> MSSIIRKIINTSKAPAAIGPYSQAVVVDRTMYVSGQLGMDPASGQLVEGGVQAQTKQALVNMGEILKEAGCGYDSVVKTTVLLADMNDFASVNDVYKTFFSSSFPARAAYQVAALPRGGLVEIEAVAVLGPLTEVS

The term Rid (reactive intermediate deaminase) refers to the hydrolytic deamination of highly reactive and labile enamines/imines to α-ketoacid and ammonia, a reaction that would be otherwise relatively slow if left to occur spontaneously. In the present study, we identified two functionally active RidA genes in the salmon genome, here named ridA-1 and ridA-2, and we performed an extensive biochemical and structural characterization of their products (SsRidA-1 and SsRidA-2). In order to better understand the structural bases of the observed differences in terms of protein stability and of enzymatic activity, the crystal structures of SsRidA-1 and SsRidA-2 were determined at 1.05 Å and at 1.36 Å resolutions, respectively. Monomeric SsRidA-1 and SsRidA-2 share the chorismate mutase-like fold common to all the members of the YjgF/YER057c/UK114 superfamily: monomers fold in a single compact domain of one six-stranded β-sheet packed against two α-helices.

Moreover, in SsRidA-1, an extra intermolecular β sheet is formed between residues Ile4-Arg6 of each monomer with the C-terminal Pro131-Val135 of the neighbouring molecule in the trimer. RidA active site has been reported to lie at the interface between monomers. In every molecule of both SsRidA-1 and SsRidA-2, an acetate molecule was visible in correspondence of Arg107 at the monomer-monomer interface (in green in Fig. 8F). Acetate ions are coordinated by the conserved residues Tyr21, Arg107 and Glu122, reported to be involved in the interaction with substrates in human RidA [hp14.5 protein, PDB: 1ONI35] and bacterial TdcF protein [PDB: 2UYN37]. The acetate molecules likely mimic the carboxylate group of RidA substrates. SsRidA-1 is an efficient catalyst with hydrophobic IA and possesses a mainly hydrophobic 15–20 loop. The conformational stability of the S. salar RidA proteins was studied by monitoring the change in ellipticity at 220 nm, which reports on the α- helical content of the proteins, by varying the temperature from 20 to 98 °C. An almost flat trace was obtained for SsRidA-1, indicating that the protein conformation was not affected in this temperature range. However, considerations concerning sequence similarity, substrate specificity, conformational stability and structural features indicate that SsRidA-1 is the bona fide functional ortholog of the vertebrate RidA. SsRidA-1 appeared to be active, like the goat enzyme, on IA derived from L-Ala, L-Met, L-Leu and L-Gln whereas SsRidA-2 was one to two orders of magnitude less active on these IA except for that derived from L-Ala, i.e. 2-iminopyruvate. Three of these sequences were ascribable to a single 137 residues-long protein, here named SsRidA-1, sharing 71% identity with HsRidA.2-methoxy-N-(4-phenyl-1,3-thiazol-2-yl)acetamide | C12 H12 N2 O2 S | 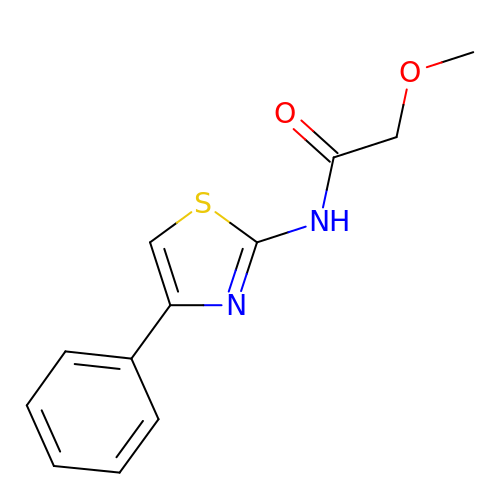ZSDPCJILFHMGQO-UHFFFAOYSA-N> EVD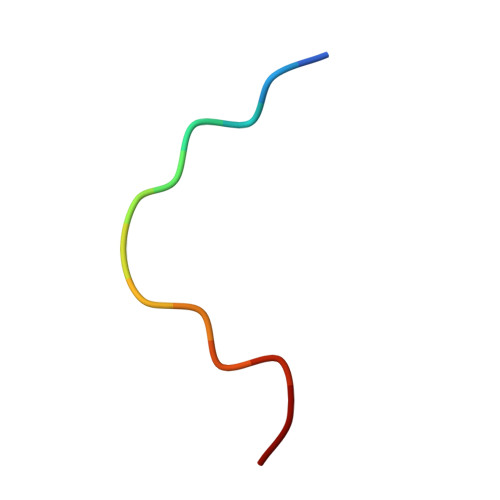LPLSDEEPSS> MFTLQANTKDQIIKDLNIGDLTIRDLNIKDLNIGDSSTVNLFKVDIPLLSNEIPLDFTFDNLPSNKKEIFESFDSFTDFVEGKTKSQESKFNPYEDNSGSTVSIRLNNSIIIAADTRHCSEMGIYSRNTSKIFRIGDFLLTITGFYADGYELYNRLKYQVQIYESFNKISIHSLANLASKIMYSKRLFPYYSYVTLSGFEGDNPYVYSFDCLGHFEEVDSVCNGSGSPLIQP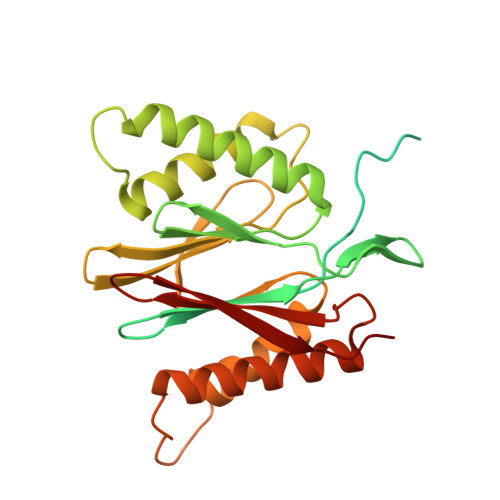LLDSTIEKKNWAGENYEVTEEYVKDIVRRGFNAASERDVKTGDNVEIWIIKKDGMTKEYERLRQD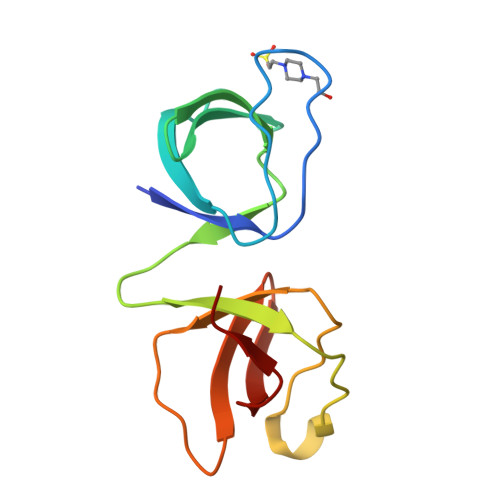> SNANTYVALYKFVPQENEDLEMRPGDIITLLEDSNEDWWKGKIQDRIGFFPANFVQRLQQNEKIFRCVRTFIGCKEQGQITLKENQICVSSEEEQDGFIRVLSGKKKGLIPLDVLENI>MGSSHHHHHHENLYFQSQWTGKPWLGKWESIDGTPENWEAFVKAANIPPKDQALYNGKQKTLLKYWKEAGEDHYHVQTSFPGTEHKMETSFKMGQEGTLSHDGVDLKYVCTEDGEQ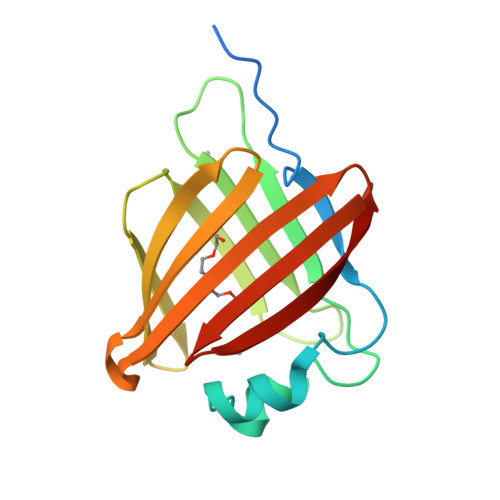LITKINIPSKNQETIVTYTATGDDLEQTFTSNGVTGKRWYKKIHA[2x]>[16x]MATGTRYAG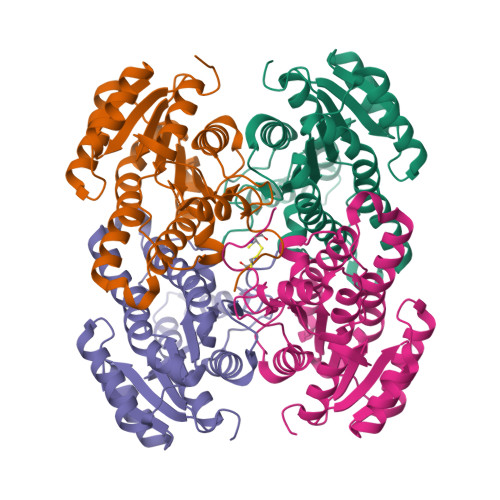KVVVVTGGGRGIGAGIVRAFVNSGARVVICDKDESGGRALEQELPGAVFILCDVTQEDDVKTLVSETIRRFGRLDCVVNNAGHHPPPQRPEETSAQGFRQLLELNLLGTYTLTKLALPYLRKSQGNVINISSLVGAIGQAQAVPYVATKGAVTAMTKALALDESPYGVRVNCISPGNIWTPLWEELAALMPDPRASIREGMLAQPLGRMGQPAEVGAAAVFLASEANFCTGIELLVTGGAELGYGCKASRSTPVDAPDIPS> MTENILRKSDEEIQKEITARVKALESMLIEQGILTTSMIDRMAEIYENEVGPHLGAKVVVKAWTDPEFKKRLLADGTEACKELGIGGLQGEDMMWVENTDEVHHVVVCTLCSCYPWPVLGLPPNWFKEPQYRSRVVREPRQLLKEEFGFEVPPSKEIKVWDSSSEMRFVVLPQRPAGTDGWSEEELATLVTRESMIGVEPAKAV;> MNGVYDVGGTDGLGPINRPADEPVFRAEWEKVAFAMFPATFRAGFMGLDEFAFGIEQMNPAEYLESPYYWHWIRTYIHHGVRTGKIDLEELERRTQYYRENPDAPLPEHEQKPELIEFVNQA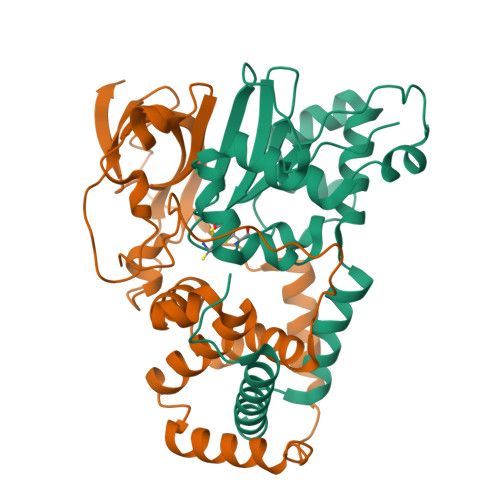VYGGLPASREVDRPPKFKEGDVVRFSTASPKGHARRARYVRGKTGTVVKHHGAYIYPDTAGNGLGECPEHLYTVRFTAQELWGPEGDPNSSVYYDCWEPYIELVDT>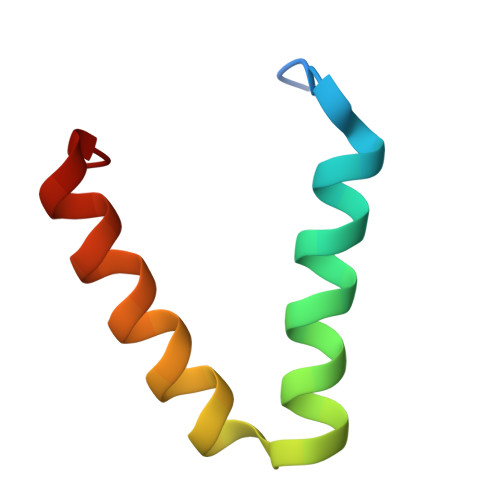 SERFPNDVDPIETRDWLQAIESVIREEGVERAQYLIDQLLAEARKGGVN> PLTSTVNGYRNVGYFAQWGVYGRAFQAKQLDVSGTAKNLTHINYSFGNINNQTLTCFMANKAQGTGPNGSDGAGDAWADFGMGYAADKSVSGKADTWDQPLAGSFNQLKQLKAKNPKLKVMISLGGWTWSKNFSKAAATEASRQKLVSSCIDLYIKGNLPNFEGRGGAGAAAGIFDGIDIDWEWPGTNSGLAGNGVDTVNDRANFKALLAEFRKQLDAYGSTNNKKYVLSAFLPANPADIDAG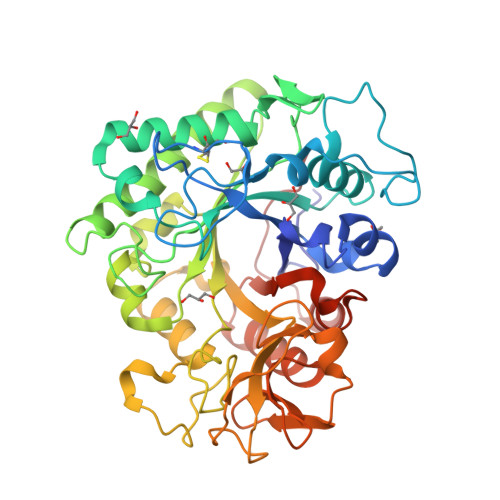GWDDPANFKSLDFGSIQGYDLHGAWNPTLTGHQANLYDDPADPRAPSKKFSADKAVKKYLAAGIDPKQLGLGLAAYGRGWTGAKNVSPWGPATDGAPGTYETANEDYDKLKTLGTDHYDAATGSAWRYDGTQWWSYDNIATTKQKTDYIVSKGLGGGMWWELSGDRNGELVGAMSDKFRAAAPGPVTEAAPP> MTTVPDLESDSFHVDWYRTYAELRETAPVTPVRFLGQDAWLVTGYDEAKAALSDLRLSSDPKKKYPGVEVEFPAYL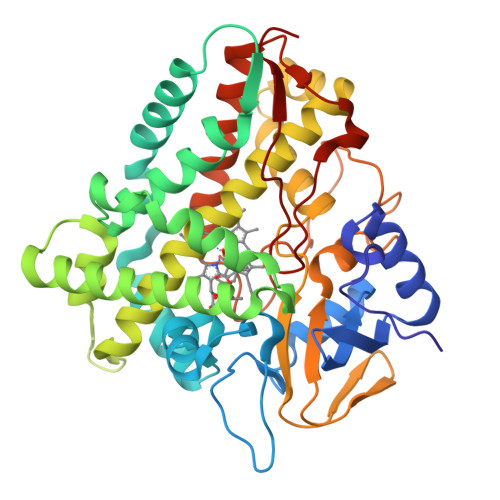GFPEDVRNYFATNMGTSDPPTHTRLRKLVSQEFTVRRVEAMRPRVEQITAELLDEVGDSGVVDIVDRFAHPLPIKVICELLGVDEKYRGEFGRWSSEILVMDPERAEQRGQAAREVVNFILDLVERRRTEPGDDLLSALIRVQDDDDGRLSADELTSIALVLLLAGFESSVSLIGIGTYLLLTHPDQLALVRRDPSALPNAVEEILRYIAPPETTTRFAAEEVEIGGVAIPQYSTVLVANGAANRDPKQFPDPHRFDVTRDTRGHLSFGQGIHFCMGRPLAKLEGEVALRALFGRFPALSLGIDADDVVWRRSLLLRGIDHLPVRLDG The structure of IDE is atypical with a very large catalytic chamber, called ‘crypt', formed by two joining N- and C-terminal domains. The zinc ion is located in the N-terminal domain, but key residues forming the hydrolytic site are located in both domains, resulting in constitution of the catalytic site only in the closed state. IDE has two substrate binding sites, one at the catalytic cleft and the other at the exosite that is distal away from the catalytic cleft. All of these results are consistent with the recognized role of IDE as major protease acting in the degradation of insulin and Aβ.

Our results show that 1,5-triazoles are much less active than the 1,4 isomers. Our structures provide the molecular basis of why compound 1 binds IDE tighter than compound 10 and 16. The 1, 4-triazole moiety allows compound 1 to complement well with the catalytic pocket of IDE, whereas 1,5-triazole makes compound 16 more compact (distance from the branching β carbon to F of compound 16 is ∼1 Å less than that of compound 1) (9.2 Å versus 10.1 Å). Compound 16 thus needs to be twisted so that only suboptimal contacts are made. The dislocation of the hydroxamate moiety from zinc ion (∼0.5 Å farther from zinc ion in 16 than that in compound 1) explains the reduced affinity. Interestingly, TGS formed the two possible triazole isomers that were shown later to display different inhibitory potencies and binding ability in enzymatic assays, crystallography and 19F NMR experiments.

>MHHHHHHAAGIPMNNPAIKRIGNHITKSPEDKREYRGLELANGIKVLLISDPTTDKSSAALDVHIGSLSDPPNIAGLSHFLEHMLFLGTKKYPKENEYSQFLSEHAGSSNAFTSGEHTNYYFDVSHEHLEGALDRFAQFFLSPLFDESAKDREVNAVDSEHEKNVMNDAWRLFQLEKATGNPKHPFSKFGTGNKYTLETRPNQEGIDVRQELLKFHSAYYSSNLMAVVVLGRESLDDLTNLVVKLFSEVENKNVPLPEFPEHPFQEEHLKQLYKIVPIKDIRNLYVTFPIPDLQKYYKSNPGHYLGHLIGHEGPGSLLSELKSKGWVNTLVGGQKEGARGFMFFIINVDLTEEGLLHVEDIILHMFQYIQKLRAEGPQEWVFQELKDLNAVAFRFKDKERPRGYTSKIAGILHYYPLEEVLTAEYLLEEFRPDLIEMVLDKLRPENVRVAIVSKSFEGKTDRTEEWYGTQYKQEAIPDEVIKKWQNADLNGKFKLPTKNEFIPTNFEILPLEKEATPYPALIKDTAMSKLWFKQDDKFFLPKANLNFEFFSPFAYVDPLHSNMAYLYLELLKDSLNEYAYAAELAGLSYDLQNTIYGMYLSVKGYNDKQPILLKKIIEKMATFEIDEKRFEIIKEAYMRSLNNFRAEQPHQHAMYYLRLLMTEVAWTKDELKEALDDVTLPRLKAFIPQLLSRLHIEALLHGNITKQAALGIMQMVEDTLIEHAHTKPLLPSQLVRYREVQLPDRGWFVYQQRNEVHNNSGIEIYYQTDMQSTSENMFLELFAQIISEPAFNTLRTKEQLGYIVFSGPRRANGIQGLRFIIQSEKPPHYLESRVEAFLITMEKSIEDMTEEAFQKHIQALAIRRLDKPKKLSAESAKYWGEIISQQYNFDRDNTEVAYLKTLTKEDIIKFYKEMLAVDAPRRHKVSVHVLAREMDSNPVVGEFPAQNDINLSQAPALPQPEVIQNMTEFKRGLPLFPLVKPHINFMAAKL[2x]>MVEIG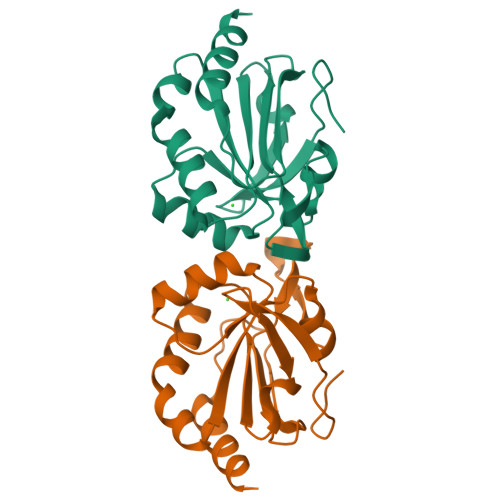EKAPEIELVDTDLKKVKIPSDFKGKVVVLAFYPAAFTSVSTKEMSTFRDSMAKFNEVNAVVIGISVDPPFSNKAFKEQNKINFTIVSDFNREAVKAYGVAGELPILKGYVLAKRSVFVIDKNGIVRYKWVSEDPTKEPNYDEIKDVVTKLSLEHHHHHH[4x]>SGQNHHEVVKFMDVYQRSYCHPIETLVDIFQEYPDEIEYIFKPSCVPLMRCGGCCNDEGLECVPTEESNITMQIMRIKPHQGQHIGEMSFLQH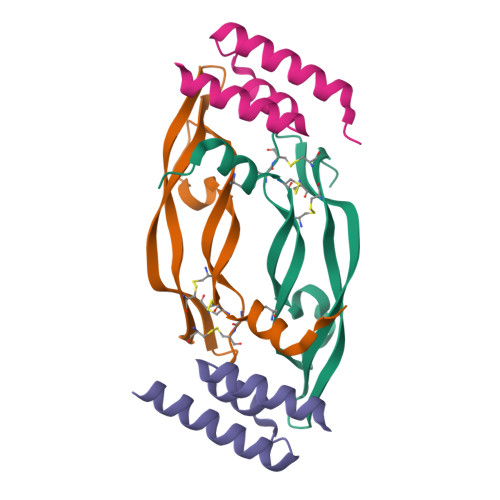NKCECRPKKD[2x];>TIDQWLLKNAKEDAIAELKKAGITEPHVISFINHAPYVSHVNGLKNAILKAHA[2x]> SNANSYVALYKFLPQENNDLALQPGDRIMLVDDSNEDWWKGKIGDRVGFF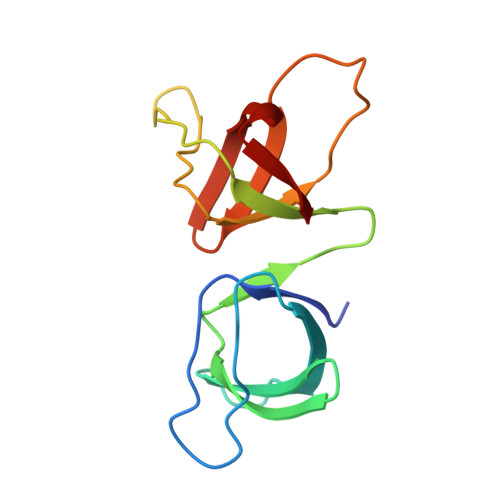PANFVQRVRPGENVWRCCQPFSGNKEQGYMSLKENQICVGVGRSKDADGFIRVSSGKKRGLVPVDALTEI> SNNGNRRNYYIAAEEISWDYSEFVQRETDIEDSDDIPEDTTYKKVVFRKYLDSTFTKRDPRGEYEEHLGILGPIIRAEVDDVIQVRFKNLASRPYSLHAHGLSYEKSSEGKTYEDDSPEWFKEDNAVQPNSSYTYVWHATERSGPESPGSACRAWAYYSAVNPEKDIHSGLIGPLLICQKGILHKDSNMPMDMREFVLLFMTFDEKKSWYYEKKSRSSWRLTSSEMKKSHEFHAINGMIYSLPGLKMYEQEWVRLHLLNIGGSQDIHVVHFHGQTLLENGNKQHQLGVWPLLPGSFKTLEMKASKPGWWLLNTEVGENQRAGMQTPFLIMDRDCRMPMGLSTGIISDSQIKASEFL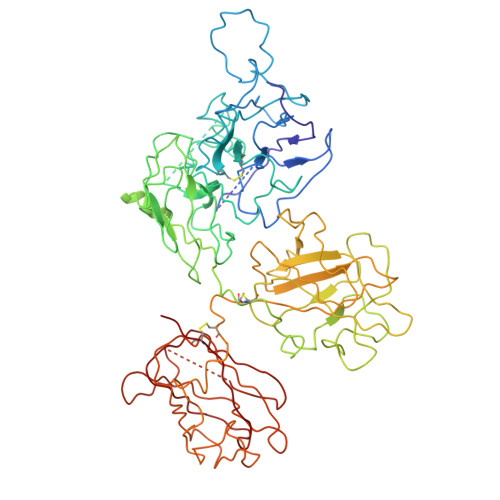GYWEPRLARLNNGGSYNAWSVEKLAAEFASKPWIQVDMQKEVIITGIQTQGAKHYLKSCYTTEFYVAYSSNQINWQIFKGNSTRNVMYFNGNSDASTIKENQFDPPIVARYIRISPTRAYNRPTLRLELQGCEVNGCSTPLGMENGKIENKQITASSFKKSWWGDYWEPFRARLNAQGRVNAWQAKANNNKQWLEIDLLKIKKITAIITQGCKSLSSEMYVKSYTIHYSEQGVEWKPYRLKSSMVDKIFEGNTNTKGHVKNFFNPPIISRFIRVIPKTWNQSIALRLELFGCDIY> FTREDYVFMAQLNENAERYDEMVETMRKISGMEGELSDKERNLLSVAYKNVIGPRRAA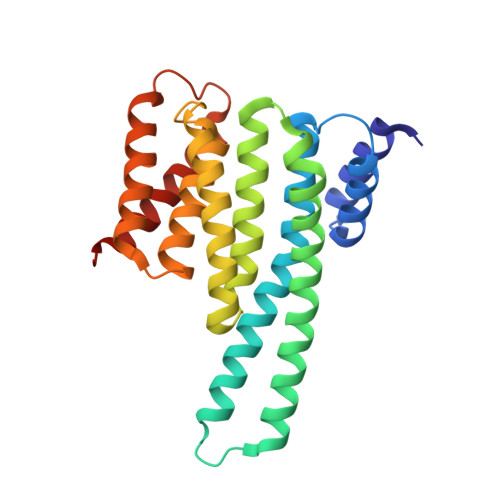WRIVSSIEAKEKGRQKPNAKRIEQIRVYRQKIEKELSDICNDILKLLQEQFVPRSTNADAKVFYYKMQGDYYRYLAEYSSGEDKEKIAGSALNAYNSAFEISQQLPPTHPIRLGLALNFSVFYYEILASPDRACELARKAFDAAITDLDKLTEESYKDSTLIMQLLRDNLNLWVTD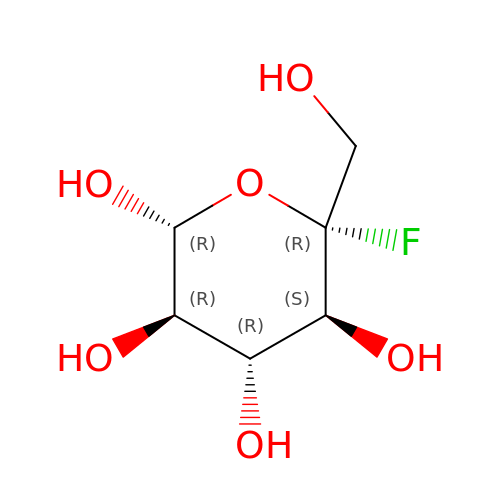5-fluoro-alpha-L-idopyranose | C6 H11 F O6 | YQZCKDSOGGIGPL-DVKNGEFBSA-N>[2x]KNRSLSVRVSTFDSELEFKLEPRASGQDLFDLVCRTIGLRESWYFGLQYVDTRSNVSWLKMEKRVRDQRVELHASNNVYVFSFYAKFFPENVSEELIQEITQHLFFLQVKQSILSMDIYCRPEASVLLASYAVHVQYGPYDYETYKDGMLAGGELLPKGVTDQYQMTPEMWEERIKTWYMDHEPMTRDEVEMEYLKIAQDLDMYGVN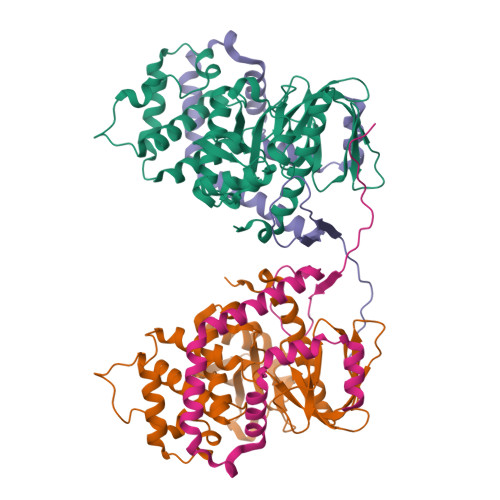YFPITNKNKTKLWLGVTSVGLNIYDERDKLTPKTTFQWNEIRHVSFDDKKFTIRLVDAKVSNFIFYSQDLHINKMILDLCKGNHDLYMRRRKPDTMEIQQ;>STNDLETAGGAELTTHSSHYLVQGDNSSGISDDFEPKEFILTDNEMEQITNEMERNHLDYLRNSKQVQSQLQTLRSEIAPHKIEENQSNLDILSEAQIKAGENKYSTLKKLKSGSTKARVAFFEEL[2x]>[6x]LAFPKEFWWGGATSGPQSEGRFAKQHRNLFDYWYEEEPDLFYDYVGPDTASDAYHQ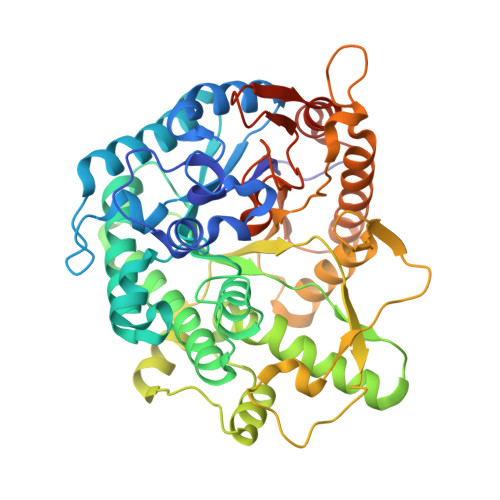IESDLTLLASLGHNSYRTSIQWTRLIDDFEQATINPDGLAYYNRVIDACLANGIRPVINLHHFDLPIALYQAYGGWESKHVVDLFVAFSKVCFEQFGDRVKDWFVHNEPMVVVEGSYLMQFHYPAIVDGKKAVQVAYNLALATAKVIQAYRRGPAELSDGRIGTILNLTPAYPASQSEADMAAAHFAELWNNDLFMEAAVHGKFPEELVAVLKKDGVLWQSTPEELALIAENRVDYLGLNFYHPKRVKAPDAIPVISPSWSPEWYYDPYLMPGRRMNVDKGWEIYPEAVYDIAIKMRDHYDNIPWFLSENGVGISGEDRYRDETGQIQDDYRIQFLKEHLTYLHKGIEAGSNCFGYHVWTPIDGWSWLNAYKNRYGLVENNIHTQVRRPKASAYWFKKVATHNRLISLEVMEEFGGSASHLSD4-[(2S)-4-[(6-aminopyridin-3-yl)sulfonyl]-2-(prop-1-yn-1-yl)piperazin-1-yl]-N-methylbenzenesulfonamide | C19 H23 N5 O4 S2 | 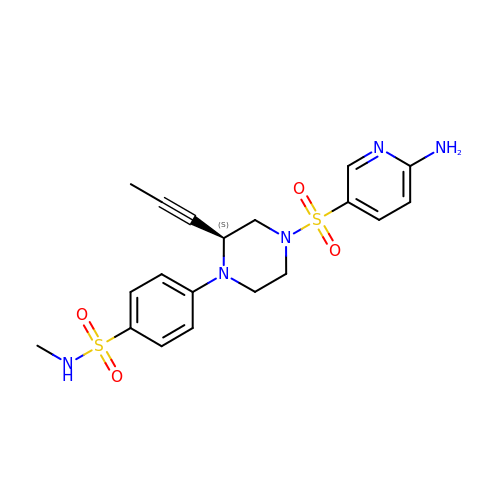AZCZVIWSFGSHOZ-INIZCTEOSA-N> QGLVPQGQTQVLQGGNKVPVVNIADPNSGGVSHNKFQQFNVANPGVVFNNGLTDGVSRIGGALTKNPNLTRQASAILAEVTDTSPSRLAGTLEVYGKGADLIIANPNGISVNGLSTLNASNLTLTTGRPSVNGGRIGLDVQQGTVTIERGGVNATGLGYFDVVARLVKLQGAVSSKQGKPLADIAVVAGANRYDHATRRATPIAAGARGAAAGAYAIDGTAAGAMYGKHITLVSSDSGLGVRQLGSLSSPSAITVSSQGE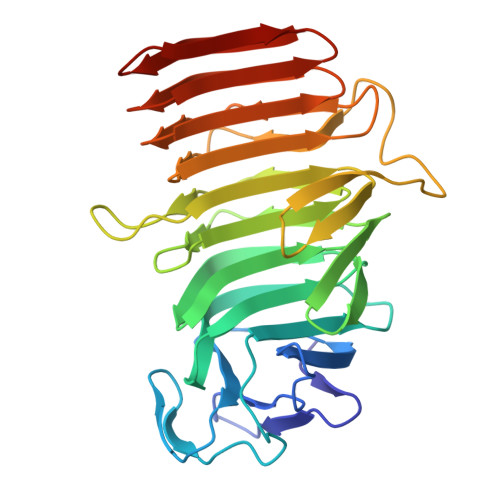IALGDATVQRGPLSLKGAGVVSAGKLASGGGAVNVAGGGAV> EEFDPELAREVEDLRQRDQVTGLLNRPTFMVALEQAVAQAGRSEGQSGFLLIEPDHYARILPEFGLDSADALIAALAAHVASVLDDSVLAARFGEHSFALLLNGNYARTHALAETVRNAFAQHVFSVGTRSATVTVSIGGVQIGEKIASIGQVLNRGTEAVRTTAELGGNAVSIYDPAAADRAEEERIERWVEQLREALVGDGFLLHYQPVLNLQGEPLELYQAFLRLERNGEMMSPNAFMAIAEEHDLVTEIDRWVVARAIRQLGERQRAGHKTHLLVRIGPNSFSDPQMIDTIREQLAVYGVPGERLWLQTPESKVFTHLRNAQQFLAAVSAMDCK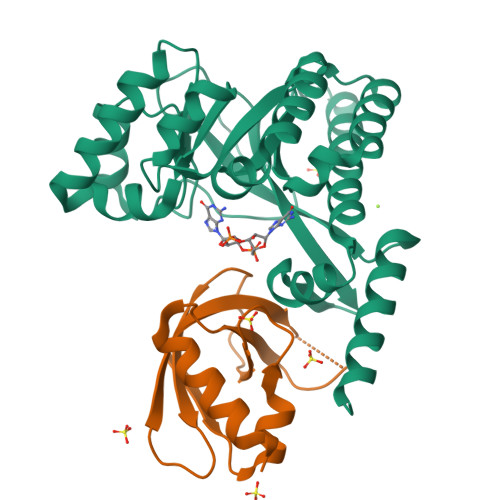VGLEQFGSGLDSFQLLAHFHPAFLKLDRGITGDIASARDSQEKIREITSRAQPAGILTMAEFVADAQSMSSFFSAGVDYVQGDFVAPTGPLMNYEFG;> MSAMNARQGILSLALKDKPALYSAYMPFVKGGGIFVPTPKRYMLGDEVFLLLTLPDSSERLPVAGKVIWTTPAGAQGNRAAGIGVQFPDGPEGEAVRNKIETLLAG> KDRISWLGQPMKIEENRTYYQKVSIDEEMLEVGDCVSVIPDDSSKPLYLARVTALWEDKNGQMMFHAHWFCAGTDTVLGATSDPLELFLVGECENMQLSYIHSKVKVIYKAPSENWAMEGGTDPETTLPGAEDGKTYFFQLWYNQEYARFESPPKTQPTEDNKHKFCLSCIRLAELRQKEMPKVLEQIEEVDGRVYCSSITKNGVVYRLGDSVYLPPEAFTFNIKVASPVKRPKKDPVNETLYPEHYRKYSDYIKGSNLDAPEPYRIGRIKEIHCGKKKGKVNEADIKLRLYKFYRPENTHRSYNGSYHTDINMLYWSDEEAVVNFSDVQGRCTVEYGEDLLESIQDYSQGGPDRFYFLEAYNSKTKNFEDPPNHARSPGNKGKGKGKGKGKGKHQVSEPKEPEAAIKLPKLRTLDVFSGCGGLSEGFHQAGISETLWAIEMWDPAAQAFRLNNPGTTVFTEDCNVLLKLVMAGEVTNSLGQRLPQKGDVEMLCGGPPCQGFSGMNRFNSRTYSKFKASLVVSFLSYCDYYRPRFFLLENVRNFVSYRRSMVLKLTLRCLVRMGYQCTFGVLQAGQYGVAQTRRRAIILAAAPGEKLPLFPEPLHVF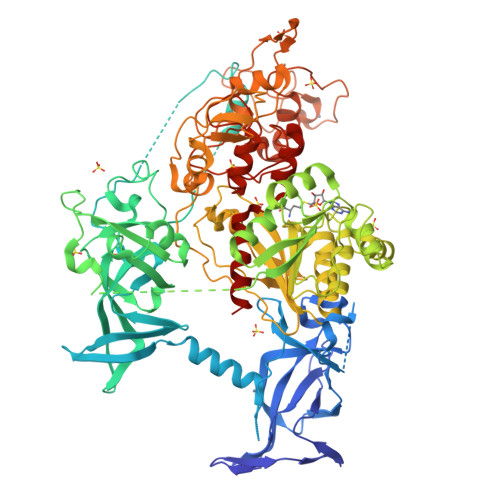APRACQLSVVVDDKKFVSNITRLSSGPFRTITVRDTMSDLPEIQNGASNSEIPYNGEPLSWFQRQLRGSHYQPILRDHICKDMSPLVAARMRHIPLFPGSDWRDLPNIQVRLGDGVIAHKLQYTFHDVKNGYSSTGALRGVCSCAEGKACDPESRQFSTLIPWCLPHTGNRHNHWAGLYGRLEWDGFFSTTVTNPEPMGKQGRVLHPEQHRVVSVRECARSQGFPDSYRFFGNILDRHRQVGNAVPPPLAKAIGLEIKLCLLSSA3-THIAOCTANOYL-COENZYME A | C28 H48 N7 O17 P3 S2 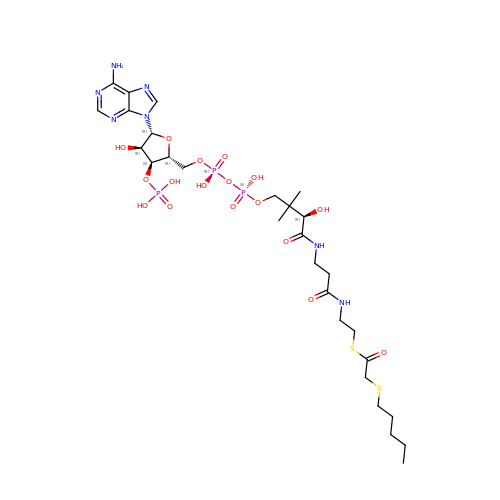| JMFXDZKFFYUOAN-SVHODSNWSA-N> MKYDTSELCDIYQEDVNVVEPLFSNFGGRASFGGQIITVKCFEDNGLLYDLLEQNGRGRVLVVDGGGSVRRALVDAELARLAV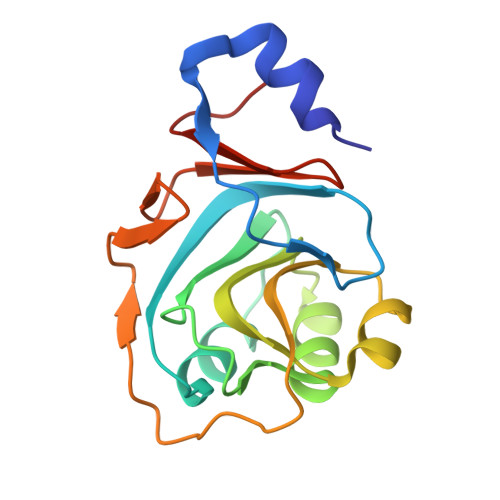QNEWEGLVIYGAVRQVDDLEELDIGIQAMAAIPVGAAGEGIGESDVRVNFGGVTFFSGDHLYADNTGIILSEDPLDIE> GMKTNEVLETIKARRSVRAYDRKQIPADDLNAILEAGAYAPSGMHYETWHFTAVCNTVKLEELNERIKGAFAKSDDKHLRERGHSETYCCYY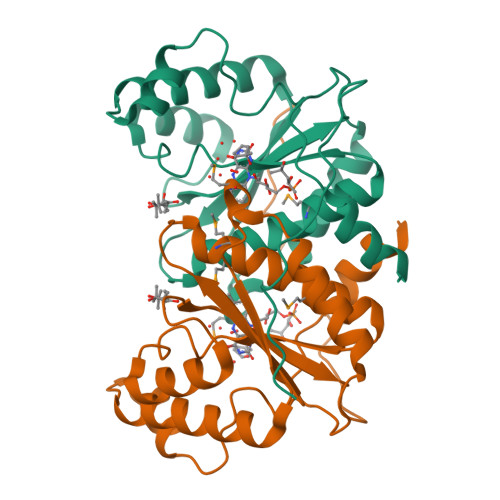HAPTLVIVSNEPKQWWAGMDCACAIENMFLAATSLGIASCWINQLGTTCDDPEVRAYLTSLGVPENHKVYGCVALGYKAEGALLKEKTVKAGTITIVE> APPRLICDSRVLERYLLEAKEAEKITTGCAEHCSLNEKITVPDTKVNFYAWKRMEVGQQAVEVWQGLALLSEAVLRGQALLVKSSQPWEPLQLHVDKAVSGLRSLTTLLRALGAQKEAISNSDAASAAPLRTITADTFRKLFRVYSNFLRGKLKLYTGEACRTGDR;>[2x]REFPPPNPDPKFESKAALLAARGPEELLCFTERLEDLVCFWEEAASAGVGPGQYSFSYQLEDEPWK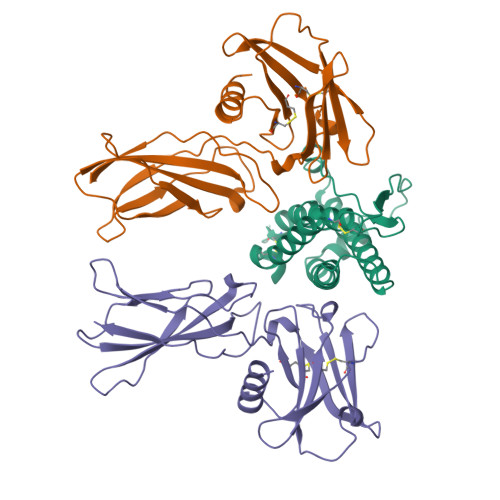LCRLHQAPTARGAVRFWCSLPTADTSSFVPLELRVTAASGAPRYHRVIHINEVVLLDAPVGLVARLADESGHVVLRWLPPPETPMTSHIRYEVDVSAGQGAGSVQRVEILEGRTECVLSNLRGRTRYTFAVRARMAEPSFGGFWSEWSEPVSLLTPSDLDP> SMSHHCEHLLERLNKQREAGFLCDC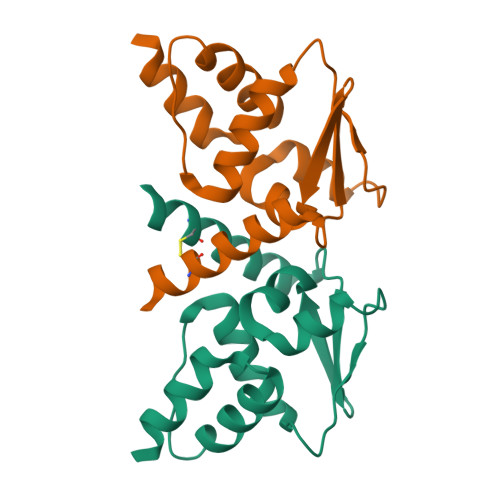TIVIGEFQFKAHRNVLASFSEYFGAIYRSTSENNVFLDQSQVKADGFQKLLEFIYTGTLNLDSWNVKEIHQAADYLKVEEVVTKCKIKMED>[3x]SIDVKYIGVKSAYVSYDVQ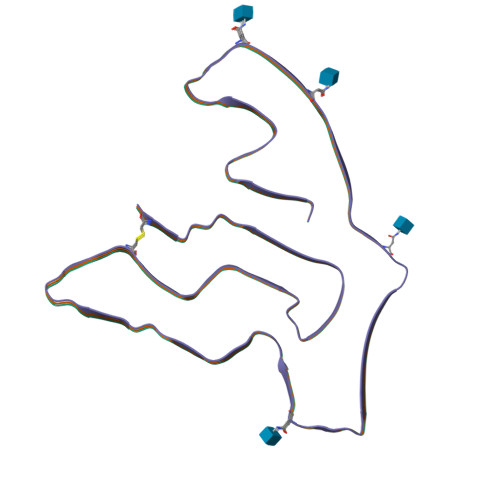KRTIYLNITNTLNITNNNYYSVEVENITAQVQFSKTVIGKARLNNISIIGPLDMKQIDYTVPTVIAEEMSYMYDFCTLISIKVHNIVLMMQVTVTTTYFGHSEQISQERYQYVDCG>[2x]MGFVNKQFNYKDPVNGVDIAYIKIPNAGQMQPVKAFKIHNKIWVIPERDTFTNPEEGDLNPPPE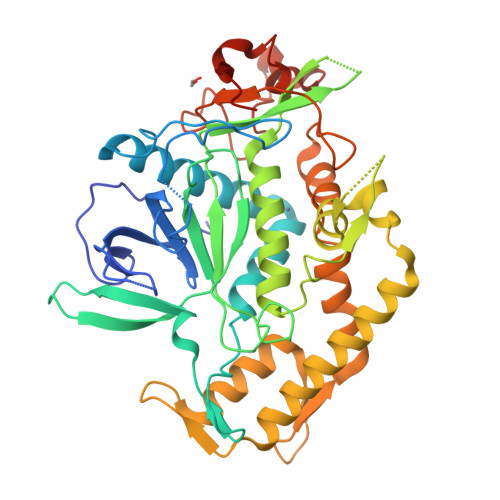AKQVPVSYYDSTYLSTDNEKDNYLKGVTKLFERIYSTDLGRMLLTSIVRGIPFWGGSTIDTELKVIDTNCINVIQPDGSYRSEELNLVIIGPSADIIQFECKSFGHEVLNLTRNGYGSTQYIRFSPDFTFGFEESLEVDTNPLLGAGKFATDPAVTLAHELIHAGHRLYGIAINPNRVFKVNTNAYYEMSGLEVSFEELRTFGGHDAKFIDSLQENEFRLYYYNKFKDIASTLNKAKSIVGTTASLQYMKNVFKEKYLLSEDTSGKFSVDKLKFDKLYKMLTEIYTEDNFVKFFKVLNRKTYLNFDKAVFKINIVPKVNYTIYDGFNLRNTNLAANFNGQNTEINNMNFTKLKNFTGLFEHHHHHH> EDELYRQSLEIISRYLREQATGAKDTKPMGRSG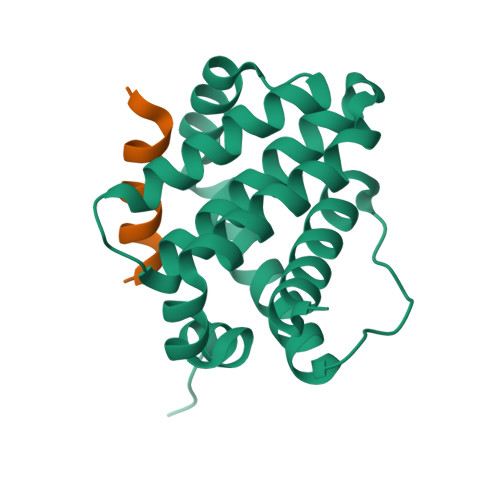ATSRKALETLRRVGDGVQRNHETAFQGMLRKLDIKNEDDVKSLSRVMIHVFSDGVTNWGRIVTLISFGAFVAKHLKTINQESCIEPLAESITDVLVRTKRDWLVKQRGWDGFVEFFHVEDLEGG;> GQVGRQLAIIGDDINR> QDNSRYTHFLTQHYDAKPQGRDDRYCESIMRRRGLTSPCQDINTFIHGNKRSIKAICENKNGNPHREN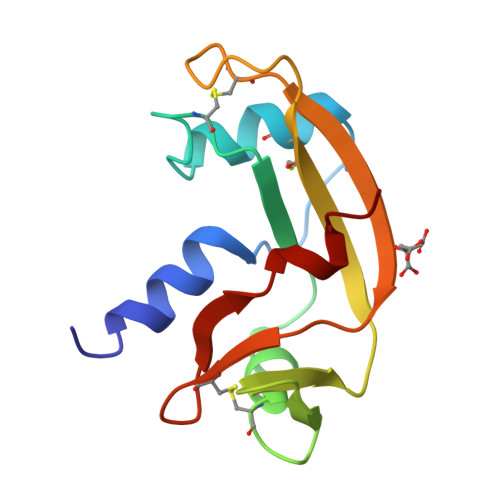LRISKSSFQVTTCKLHGGSPWPPCQYRATAGFRNVVVACENGLPVHLDQSIFRRP>ADTIVAVELDTYPNTDIGDPNYPHIGIDIKSVRSKKTAKWNMQNGKVGTAHIIYNSVGKRLSAVVSYPNGDSATVSYDVDLDNVLPEWVRVGLSASTGLYKETNTILSWSFTSKLKSNSTHETNALHFMFNQFSKDQKDLILQGDATTGTDGNLELTRVSSNGSPQGSSVGRALFYAPVHIWESSAVVASFDATFTFLIKSPD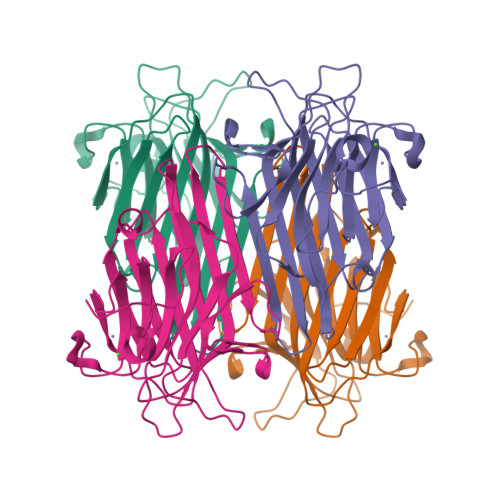SHPADGIAFFISNIDSSIPSGSTGRLLGLFPDAN[4x]> AVNIVDYSDCFEGISGGAIFCNTKNKEYNIYNKELIETRRSPCSTFKIVSTLIGLEKGVINSKESVMGYDGTDYPNKNWNKNLSLEEAFKESCVWYYKKLINKVDAKSVQNILDDLKYGNCDIS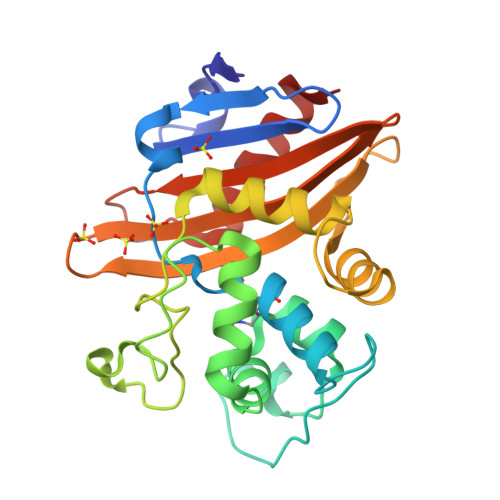EWEGDLKNGKGHLNGFWLESSLQISPKEQVQTMAKIFEGDTNFKKEHINILRDIMAIDVNDANINVYGKTGTGFDEKNKRVDAWFVGMLEREGDTYYFAIKSDDSNKEITGPKVKEIAINIIKKYYS>MANKQQNFNTGIKDFDFWLSEVEALLASEDYGKDLASVNNLLKKHQLLEADISAHEDRLKDLNSQADSLMTSSAFDTSQVKDKRETINGRFQRIKSMAAARRAKLNESHR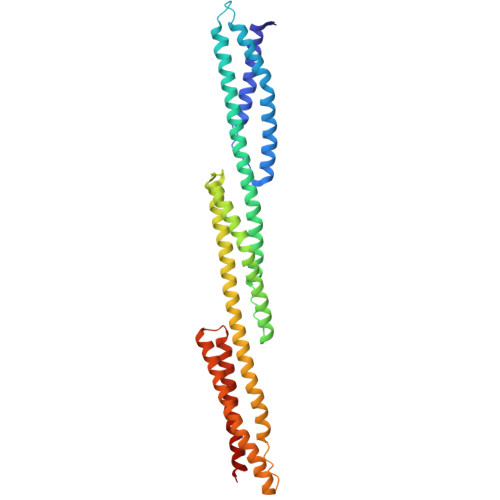LHQFFRDMDDEESWIKEKKLLVSSEDYGRDLTGVQNLRKKHKRLEAELAAHEPAIQGVLDTGKKLSDDNTIGKEEIQQRLAQFVDHWKELKQLAAARGQRLEESLEYQQFVANVEEEEAWINEKMTLVASEDYGDTLAAIQGLLKKHEAFETDFTVHKDRVNDVCANGEDLIKKNNHHVENITAKMKGLKGKVSDLEKAAAQRKAKLDENSA[2x]>MHRTSNGSHATGGNLPDVASHYPVAYEQTLDGTVGFVIDEMTPERATASVEVTDTLRQRWGLVHGGAYCALAQMLATEATVAVVHEKGMMAVGQSNHTSFFRPVKEGHVRAEAVRIHAGSTTWFWDVSLRD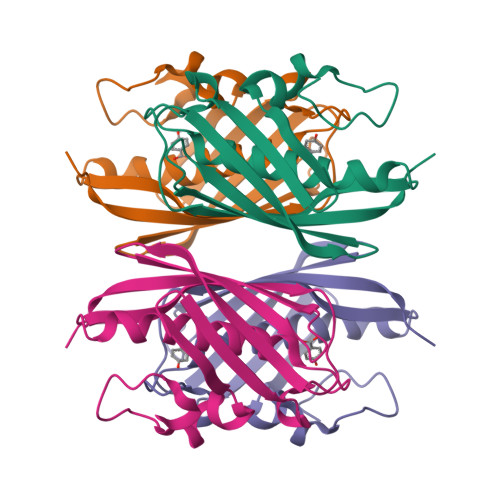DAGRLCAVSSMSIAVRPRRD[2x]>EDDEDYGDLGGCPFLVAENKTG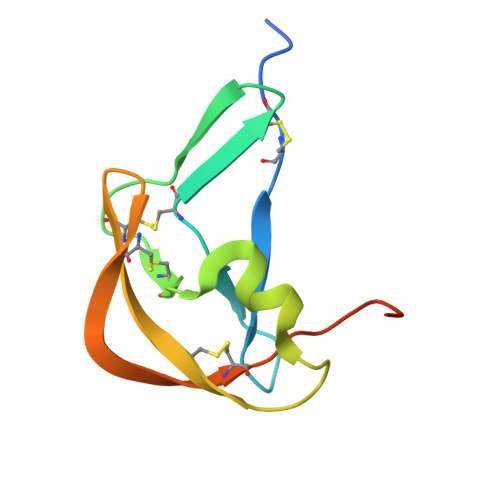YPTIVACKQDCNGTTETAPNGTRCFSIGDEGLRRMTANLPYDCPLGQCSNGDCIPKETYEVCYRRNWRDKKNHHHHHH[2x]> MLLVKAVKVLVMGGCMLPIAFGALGTGVLFAGFN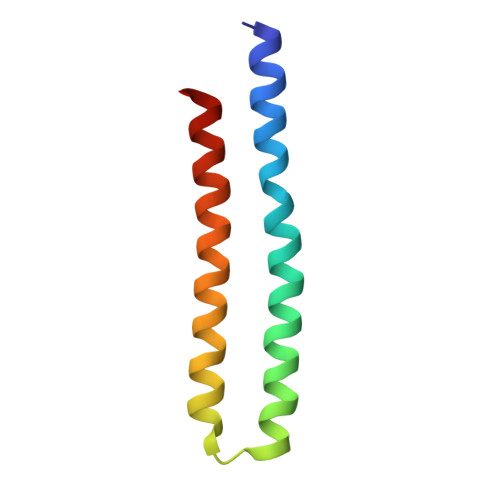VALSRNPEETESLFNNTLMGFALIETFIFMSIGLGFFVLFAA>[2x]GHMPLPTELARHLTEEKIAFVQRSGLRA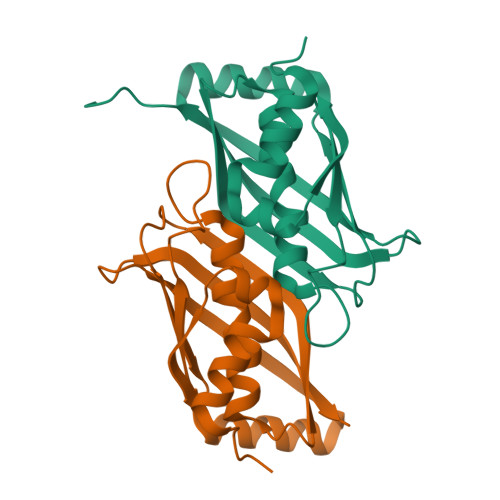EVLEPGYVRLRMPGAGNENHIGSMYAGALFTLAELPGGALFLTSFDSARFYPIVKEMTLRFRRPAKGDIRVEARLDAERIRQLETEAGERGKAEYSLELQLTDEQGEVVAESAALYQLRSHARPGS>[2x]HMAKSLPLNSRSKTTALKQPRELFSYARDIDGKYVYDDPENSLSYYYLPDSTIDTGIDL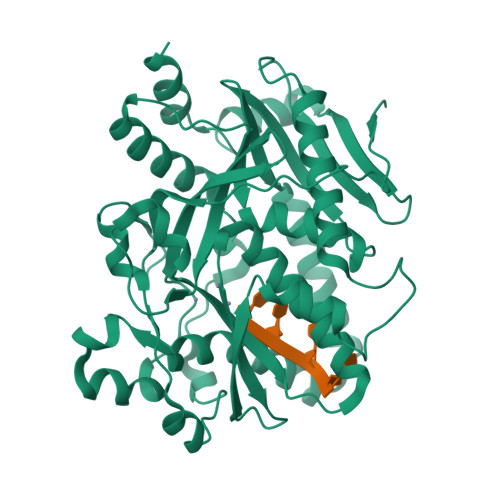QGGYSKFKKIPDEQNLADFNSLLKAIIKYETSEGKKISSDIITFREIMTKILSLPYNLTDPIDLYVVPFDGQLFIKSDDELDMKRRKEQEVRMKQTNTVERYDYMKRCEYVGYKFETIATIPKPWSQVSRSQIENRNKKVVNNYEQYLSVIRTGIGNVKLVLAGEIDCCWDYLPDEQNKKLNHYVELKTSRIIENNSQVVSFEQKLFKAWCQCFLMGVTKIIYGFRDNNLILKNVELFNTEEIPILIKNNPLTNAATEKKINCTNALKWYGAVVDWLNTTVDKKDEIKSYRLKYDPVRKSFTLSETDSETNEKLRNGQLLTPEFTEWRQSLKK>GRKERERLEEKLEDANERIAELVKLEERQRIARDLHDTLGQKLSLIGLKSDLARKLIYKDPEQAARELKSVQQTARTSLNEVRKIVSSMKGIRLKDELINIKQILEAADIMFIYEEEKWPENISLLNENILSMCLKEAVTNVVKHSQAKTCRVDIQQLWKEVVITVSDDGTFKGEENSFSKGHGLLGMRERLEFANGSLHIDTE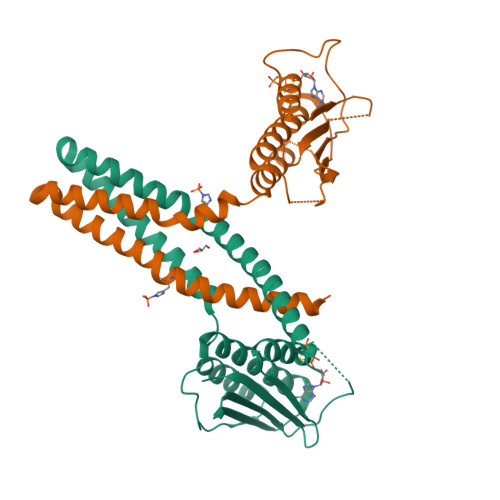NGTKLTMAIPNNSK[2x]>[4x]TLLRNFGNVYDNPVLLDRSVTAPVTEGFNVVLASFQALYLQYQKHHFVVEGSEFYSLHEFFNESYNQVQD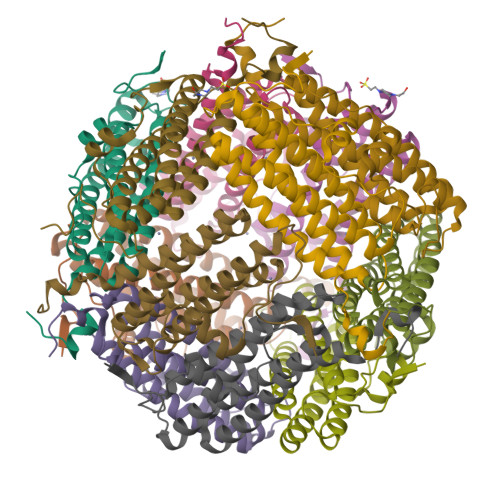HIHEIGERLDGLGGVPVATFSKLAELTCFEQESEGVYSSRQMVENDLAAEQAIIGVIRRQAAQAESLGDRGTRYLYEKILLKTEERAYHLSHFLAKDSLTLGFVQAA We have unraveled structures of the soluble components and the pore assembly of the YaxAB cytolysin from Y. enterocolitica. The crystal structures show an atypical fold, comprising a head domain reminiscent of ClyA family toxins and pronounced coiled-coil and foot domains unique to the YaxAB system. In line with our finding that the isolated YaxA and YaxB head domains form spoked oligomers in solution, the YaxB head domain in isolation was sufficient for recruitment to membrane-bound YaxA. Together, our biochemical data support a role for YaxA as the initial membrane-interacting subunit of the toxin, able to bring the lytic effector YaxB to the target cell surface. Therefore, we propose that this class of toxins defines a new structural family of α-PFTs.

The orthologue PaxB produced better diffracting crystals than YaxB and thus served as template for molecular replacement phasing (the two proteins share 40% amino acid sequence identity, whereas YaxA shares 18% and 22% sequence identity with PaxB and YaxB, respectively). Our structural data confirmed that YaxB is a true homolog to PaxB, with a RMSD of 2.1 Å across 210 Cα pairs. Notably, the YaxB foot domain could not be resolved in the 2Fo–Fc electron density map and therefore remains unmodeled. Because our monomeric YaxB model was incomplete (with the foot domain not resolved in the electron density map), we superposed both monomeric YaxB and PaxB coordinates with protomeric YaxB. This likewise revealed only small conformational changes in the YaxB head domain (RMSD of 1.3 Å across 178 Cα pairs), accompanied by a slight movement of the coiled-coil stalk away from the incoming YaxA. Using a liposome float assay, we could establish that YaxA binds membranes while YaxB fails to do so.

> GAEISTFPHSGLSYPDINFKIFSQGVKNISHLAQFKTTGVEVLQEKALRVSLYSQRLDVIVRESLSSLQVKLENTLALTYFTTLEEIDEALISQDIDEESKSEMRKERINIIKNLSNDITQLKQLFIEKTELLDKSSSDLHNVVIIEGTDKVLQAEQLRQKQLTEDIATKELERKEIEKKRDKIIEALDVIREHNLVDAFKDLIPTGENLSELDLAKPEIELLKQSLEITKKLLGQFSEGLKYIDLTDARKKLDNQIDTASTRLTELNRQLEQSEKLIAGVNAVIKIDQEKSAVVVEAEKLSRAWHIFIHEITALQGTSLNEVELSKPLIKQQIYLESLIKQLI>[4x]KHSLPDLPYDYGALEPHINAQIMQLHHSKHHAANVNNLNVTEEKYQEAL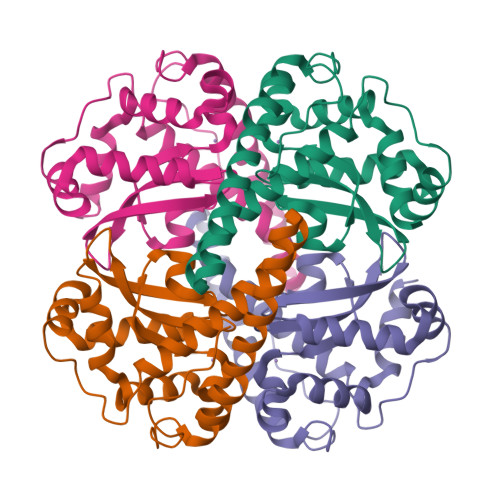AKGDVTAQIALQPALKFNGGGHINHSIFWTNLSPNGGGEPKGELLEAIKRDFGSFDKFKEKLTAASVGVQGSGWGWLGFNKERGHLQIAACPNQDPLQGTTGLIPLLGIDVWEHAYYLQYKNVRPDYLKAIWNVINWENVTERYMACKK> GFKTFYIKVILKEGTQLKSARIYLVFHKLEELKCEVVRTIPSVEEIEEEKFENEVEL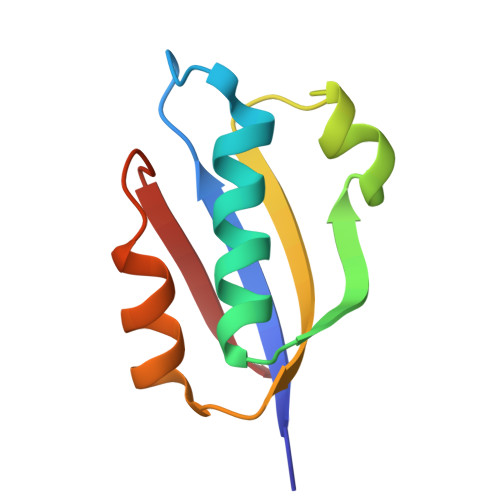FVISPVDLEKLSEALSSIADIERVIIKEV>[8x]SNAMSPIIAPPAELVDPKDRVQLRRVFGDFPTGVTVVTVGGSEPRGMTANSFTSVSLSPPLVLICVGKDAVMHQRLTALPTFAVSVLEAGQEKAARHFADHSHPP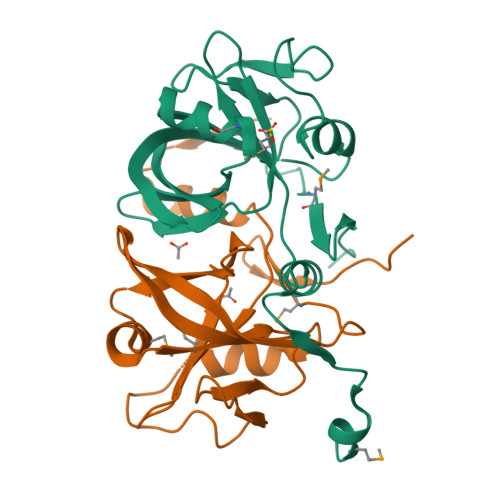GVDQFDTVDWVLGEESGAPLIAGAVAHLECAIHRLYEGGDHTIFLGEVITATRWPAREGMLFSGGRFRRFAPDADEGRAA> MKDLVDTTEAYLRTIYELEEEGVTPLRARIAERLEQSGPTVSQTVARMERDGLVVVASDRSLQMTPTGRTLATAVMRKHRLAERLLTDIIGLDINKVHD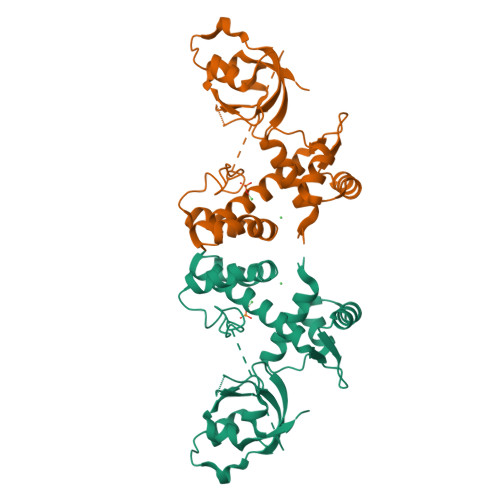EADRWEHVMSDEVERRLVKVLKDVSRSPFGNPIPGLDELGVGNSDAAAPGTRVIDAATSMPRKVRIVQINEIFQVETDQFTQLLDADIRVGSEVEIVDRDGHITLSHNGKDVELLDDLAHTIRIEEL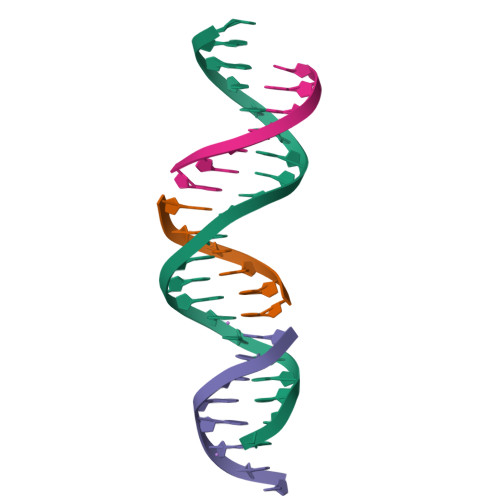> GAGCAGACTTGACGACACTCA;> TCGTCA;> TCTGAGTG;> AGTCTGC>[3x]MSDPHSSPLLPEPLSSRYKLYEAEFTSPSWPSTSPDTHPALPLLEMPEEKDLRSSNEDSHIVKIEKLNERSKRKDDGVAHRDSAGQRCICLSKAVGYLTGDMKEYRIWLKDKHLALQFIDWVLRGTAQVMFINNPLSGLIIFIGLLIQNPWWTITGGLGTVVSTLTALALGQDRSAIASGLHGYNGMLVGLLM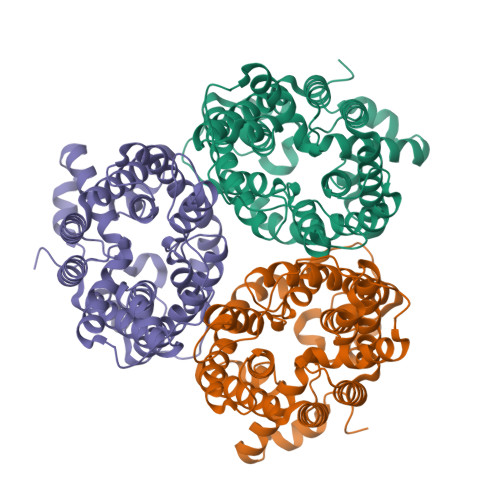AVFSEKLDYYWWLLFPVTFTAMSCPVLSSALNSIFSKWDLPVFTLPFNIAVTLYLAATGHYNLFFPTTLVEPVSSVPNITWTEMEMPLLLQAIPVGVGQVYGCDNPWTGGVFLVALFISSPLICLHAAIGSIVGLLAALSVATPFETIYTGLWSYNCVLSCIAIGGMFYALTWQTHLLALICALFCAYMEAAISNIMSVVGVPPGTWAFCLATIIFLLLTTNNPAIFRLPLSKVTYPEANRIYYLTVKSGEEEKAPSG>[2x]KPLQNWEQASPGENAHSSLGLSGAGEEGVFDLQMFLENMKVDFLRSLNLSGIPSQDKTRAEPPQYMIDLYNRYTTDKSSTPASNIVRSFSVEDAISTAATEDFPFQKHILIFNISIPRHEQITRAELRLYVSCQNDVDSTHGLEGSMVVYDVLEDSETWDQATGTKTFLVSQDIRDEGWETLEVSSAVKRWVRADSTTNKNKLEVTVQSHRESCDTLDISVPPGSKN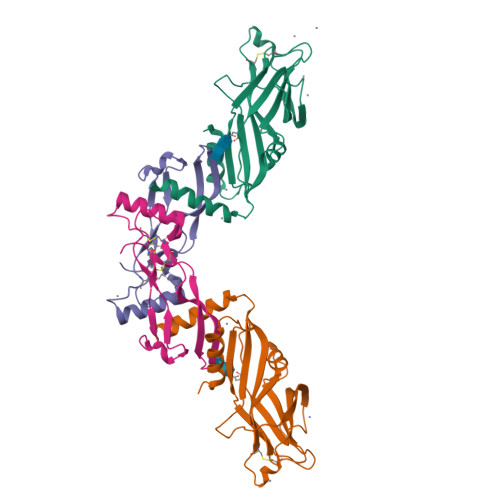LPFFVVFSNDRSNGTKETRLELKEMIGHEQETMLVKTAKNAYQVAGESQEEEGLDGYTAVGPLLARRKR;>SAGAGSHCQKTSLRVNFEDIGWDSWIIAPKEYEAYECKGGCFFPLADDVTPTKHAIVQTLVHLKFPTKVGKACCVPTKLSPISVLYKDDMGVPTLKYHYEGMSVAECGCR[2x]>[4x]KLPYVGDKEPL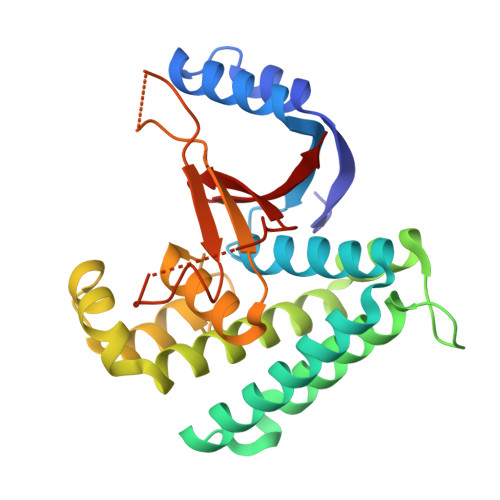STLAAEFQSGSPILQEKIKLLGEQYDALRRTRGDGNCFYRSFMFSYLEHILETQDKAEVERILKKIEQCKKTLADLGYIEFTFEDFFSIFIDQLESVLQGHESSIGAEELLERTRDQMVSDYVVMFFRFVTSGEIQRRAEFFEPFISGLTNSTVVQFCKASVEPMGEESDHVHIIALSDALGVPIRVMYLDRSSCDAGNISVNHHDFSPEANSSDGAAAAEKPYITLLYRPGHYDILYPK> GAMGSGIQRPSAVTSMTRTRDVMQLWSLLEACLQSNLMKRAFSILESLYLVPEHKQRFIEDYNMYLNSFSKNDPNFPILKMNEKLTNDLETSFKDVNYNDKTLAIMIHHALNFHSTTSSMLLKPIISAYLKMSVNGIREIFSCLDILTISDLNILMNDLKVITPSQLPNSVRPILESLTLSPTPVNNIENEEGLNKVEAENDSKLHKASNASSDSIKKPSLDPLREVSFHGSTEVLSKDAEKLIAVDTIGMRVIRHTLLGLSLTPEQKEQISKFKFDANDNVLKMKPTKNDDNNNSINFFEIYNSLPTLEEKKAFESALNIFNQDRQKVLENRATEAARERWKHDFEEAKARGDISIEKNLNVKLWKWYNEMLPLVKEEINHCRSLLSEKLSDKKGLNKVDTNRLGYGPYLTLIDPGKMCVITILELLKLNSTGGVIEGMRTARAVISVGKAIEMEFRSEQVLKSESQAFRDVNKKSPEFKKLVQNAKSVFRSSQIEQSKILWPQSIRARIGSVLISMLIQVAKVSVQGVDPVTKAKVHGEAPAFAHGYQYHNGSKLGVLKIHKTLIRQLNGERLIASVQPQLLPMLV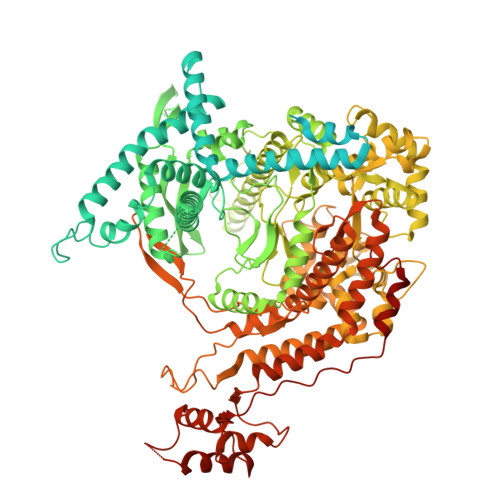EPKPWVNWRSGGYHYTQSTLLRTKDSPEQVAYLKAASDNGDIDRVYDGLNVLGRTPWTVNRKVFDVVSQVWNKGEGFLDIPGAQDEMVLPPAPPKNSDPSILRAWKLQVKTIANKFSSDRSNRCDTNYKLEIARAFLGEKLYFPHNLDFRGRAYPLSPHFNHLGNDMSRGLLIFWHGKKLGPSGLKWLKIHLSNLFGFDKLPLKDRVAFTESHLQDIKDSAENPLTGDRWWTTADKPWQALATCFELNEVMKMDNPEEFISHQPVHQDGTCNGLQHYAALGGDVEGATQVNLVPSDKPQDVYAHVARLVQKRLEIAAEKGDENAKILKDKITRKVVKQTVMTNVYGVTYVGATFQIAKQLSPIFDDRKESLDFSKYLTKHVFSAIRELFHSAHLIQDWLGESAKRISKSIRLDVDEKSFKNGNKPDFMSSVIWTTPLGLPIVQPYREESKKQVETNLQTVFISDPFAVNPVNARRQKAGLPPNFIHSLDASHMLLSAAECGKQGLDFASVHDSYWTHASDIDTMNVVLREQFIKLHEVDLVLRLKEEFDQRYKNYVKIGKLKRSTDLAQKIIRIRKDLSRKLGRSTTLADEIYFEKKRQELLNSPLIEDRNVGEKMVTTVSLFEDITDLDALELENGGDENSGMSVLLPLRLPEIPPKGDFDVTVLRNSQYFFS>VDFHGYARSGIGWTGSGGEQQCFQTTGAQSKYRLGNECETYAELKLGQEVWKEGDKSFYFDTNVAYSVAQQNDWEATDPAFREANVQGKNLIEWLPGSTIWAGKRFYQRHDVHMIDFYYWDISGPGAGLENIDVGFGKLSLAATRSSEAGGSSSFASNNIYDYTNETANDVFDVRLAQMEINPGGTLELGVDYGRANLRDNYRLVDGASKDGWLFTAEHTQSVLKGFNKFVVQYATDSMTSQGKGLSQGSGVAFDNEKFAYNINNNGHMLRILDHGAISMGDNWDMMYVGMYQDINWDNDNGTKWWTVGIRPMYKWTPIMSTVMEIGYDNVESQRTGDKNNQYKITLAQQWQAGDSIWSRPAIRVFATYAKW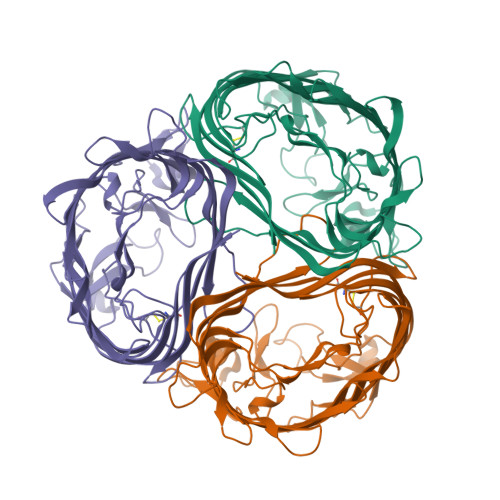DEKWGYDYTGNADNNANFGKAVPADFNGGSFGRGDSDEWTFGAQMEIWW[3x]4-{[methyl(3-{[7-propyl-3-(trifluoromethyl)-1,2-benzisoxazol-6-yl]oxy}propyl)carbamoyl]amino}benzoic acid | C23 H24 F3 N3 O5 | 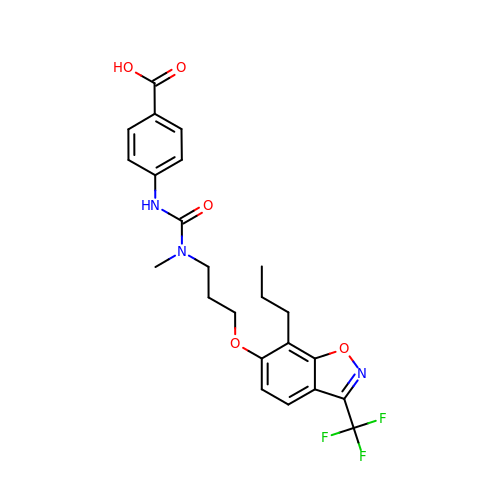JBWDFALEPSJCLA-UHFFFAOYSA-N>MGSSHHHHHHSSGLQGTENLYFQSHMAAATGGLTPEQIIAVDGAHLWHPYSSIGREAVSPVVAVAAHGAWLTLIRDGQPIEVLDAMSSWWTAIHGHGHPALDQALTTQLRVMNHVMFGGLTHEPAARLAKLLVDITPAGLDTVFFSDSGSVSVEVAAKMALQYWRGRGLPGKRRLMTWRGGYHGDTFLAMSICDPHGGMHSLWTDVLAAQVFAPQVPRDYDPAYSAAFEAQLAQHAGELAAVVVEPVVQGAGGMRFHDPRYLHDLRDICRRYEVLLIFDEIATGFGRTGALFAADHAGVSPDIMCVGKALTGGYLSLAATLCTADVAHTISAGAAGALMRGPTFMANPLACAVSVASVELLLGQDWRTRITELAAGLTAGLDTARALPAVTDVRVCGAIGVIECDRPVDLAVATPAALDRGVWLRPFRNLVYAMPPYICTPAEITQITSAMVEVA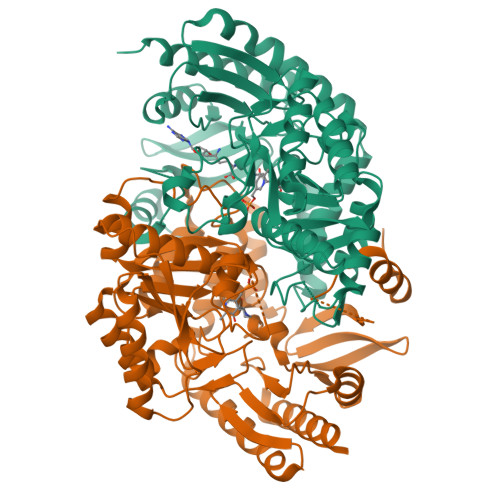RLVGSLP[2x]> MRTFFVGGNWKANPKTVEEAEKLIEMLNGAKVEGNVEVVVAAPFVFLPTLQQKLRKDWKVSAENVFTKPNGAFTGEVTVPMIKSFGIEWTILGHSERRDILKEDDEFLAAKAKFALENGMKIIYCCGEHLSEREAGKA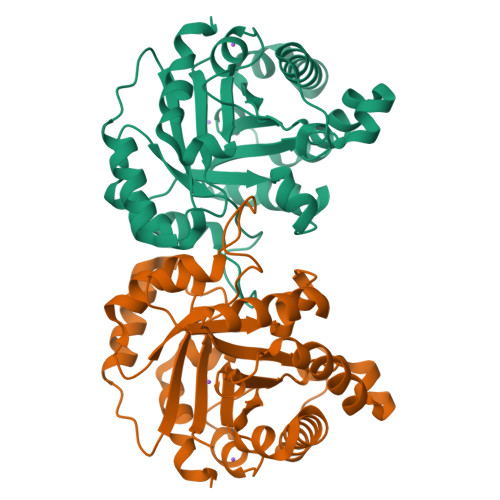SEFVSAQIEKMIPAIPAGKWDDVVIAYEPIWAIGTGKVASTQDAQEMCKVIRDILAAKVGADIANKVRILYGGSVKPNNCNELAACPDVDGFLVGGASLEPGFINIVNSNVHSK methyl 5-amino-6-(7-amino-6-methoxy-5,8-dioxo-5,8-dihydroquinolin-2-yl)-4-(2-hydroxy-3-methoxyphenyl)-3-methylpyridine-2-carboxylate | C25 H22 N4 O7 | 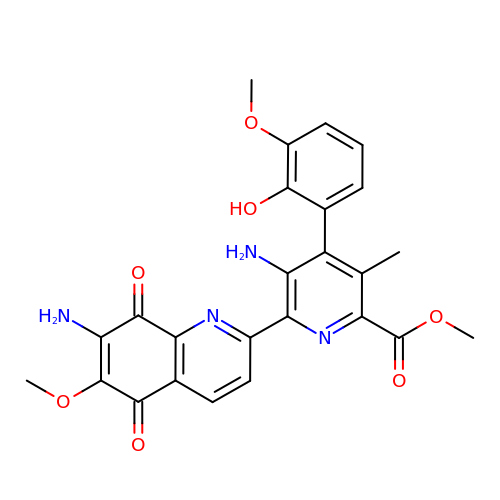OQVKIMFXFHBJLD-UHFFFAOYSA-N(3~{R})-3-azanylazepan-2-one | C6 H12 N2 O | 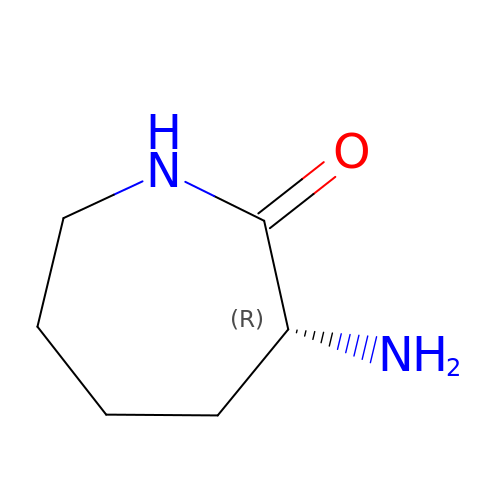BOWUOGIPSRVRSJ-RXMQYKEDSA-N> VHINKGGRPRQHLLSLTRRAQKHRLRELKIQVKEFADKEEGGDVKAVCLTLFLLALRARNEHRQADELEAIMQGRGSGLQPAVCLAIRVNTFLSCSQYHKMYRTVKAITGRQIFQPLHALRNAEKVLLPGYHPFEWQPPLKNVSSRTDVGIIDGLSGLASSVDEYPVDTIAKRFRYDSALVSALMDMEEDILEGMRSQDLDDYLNGPFTVVVKESCDGMGDVSEKHGSGPAVPEKAVRFSFTVMRITIEHGSQNVKVFEEPKPNSELCCKPLCLMLADESDHETLTAILSPLIAEREAMKSSELTLEMGGIPRTFKFIFRGTGYDEKLVR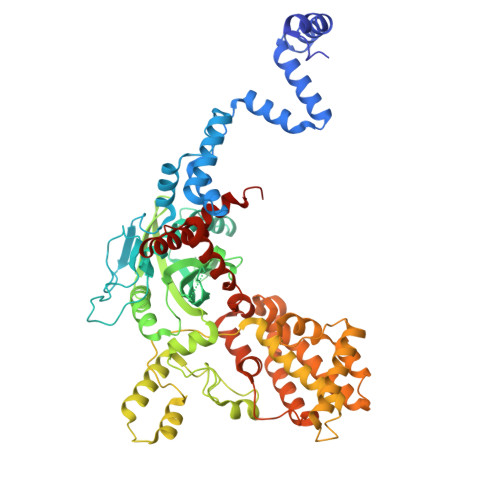EVEGLEASGSVYICTLCDTTRLEASQNLVFHSITRSHAENLQRYEVWRSNPYHESVEELRDRVKGVSAKPFIETVPSIDALHCDIGNAAEFYKIFQLEIGEVYKHPNASKEERKRWQATLDKHLRKRMNLKPIMRMNGNFARKLMTQETVDAVCELIPSEERHEALRELMDLYLKMKPVWRSSCPAKECPESLCQYSFNSQRFAELLSTKFKYRYEGKITNYFHKTLAHVPEIIERDGSIGAWASEGNQSGNKLFRRFRKMNARQSKCYEMEDVLKHHWLYTSKYLQKFMNAHNA> SALAEGQSCG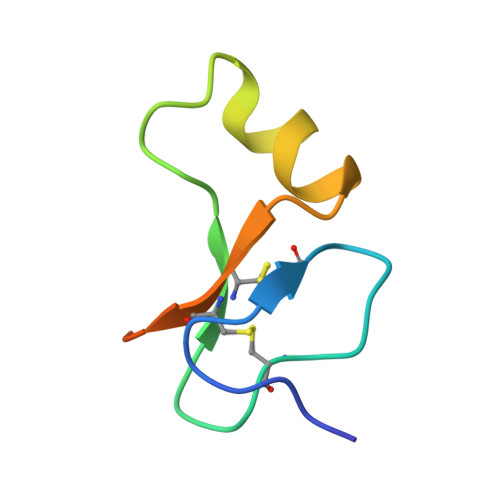VYTERCAQGLRCLPRQDEEKPLHALLHGRGVCLNEKSYREQVKI>[2x]MNLHVCALALLLFGSIATVRGRAVDLVDDSNDVDN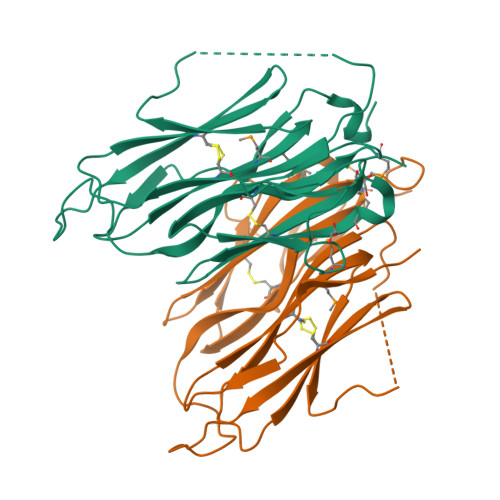SIEAEEEKPRNRAFEADWLKFTKTPPTKLQQADGATIEIVCEMMGSQVPSIQWVVGHLPRSELDDLDSNQVAEEAPSAIVRVRSSHIIDHVLSEARTYTCVGRTGSKTIYASTVVHPPRSSRLTPEKTYPGAQKPRIIYTEKTHLDLMGSNIQLPCRVHARPRAEITWLNNENKEIVQGHRHRVLANGDLLISEIKWEDMGNYKCIARNVVGKDTADTFVYPVLNEEDEVLFQ>EVEEKSKDVINFTAE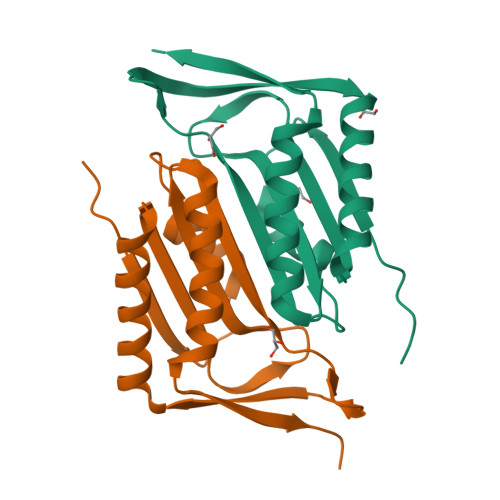KLSVDEVSQLVISPLCGAISLFVGTTRNNFEGKKVISLEYEAYLPMAENEVRKICSDIRQKWPVKHIAVFHRLGLVPVSEASIIIAVSSAHRAASLEAVSYAIDTLKAKVPIWKKEIYEE[4x]> GKELHESSTIISFKEHTDVNADSILELSFLKLQTKDSCLVKNVGLIRELNNCLLILDSANSNLYVFNKSGAFVNQIGQKGSGPGEYILLSSFFVDNNKNYIAAIDIAQDKVLYYNATDFSFLYERRLPFSTSCCLQLEDGNLLWNSREYTDSKLSDFYFVVTDSLFDIIDYKMNKEFKSGYTTGPSQMIYKVGTNVFAYTPFDLTIYRVGTSEIVPAHSFSFEGTDIPSLDFLNKTSNQGNSNYLYDLIQSDYISYYCVEETERDLFVCYMKNKEKYIGLYDKNTDRT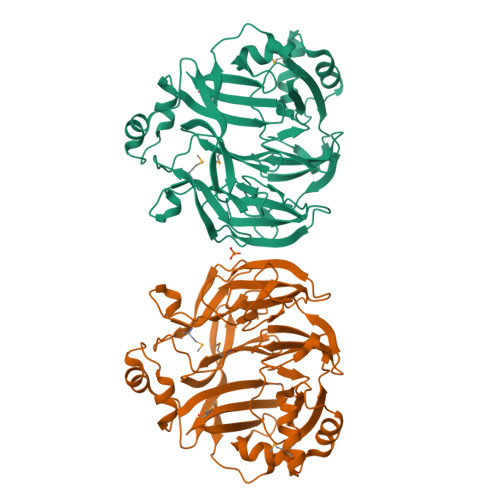YNYPIKIFQDQLKVGELNYFSIGSVDDYHVAPLDVLSLKDMAGNGYVFDDKLSELLTISNEEDNSILLFVRIKK>KQLRLYQLYSRTSGKHIQVLGRRISARGEDGDKYAQLLVETDTFGSQVRIKGKETEFYLCMNRKGKLVGKPDGTSKECVFIEKVLENNYTALMSAKYSGWYVGFTKKGRPRKGPKTRENQQDVHFMKRYPKGQPELQKPFK[4x]

Fibroblast growth factors (FGFs) regulate a plethora of critical processes in development. These processes are mediated by signaling through four FGF receptors (FGFR1–4), which are high-affinity cell surface receptor tyrosine kinases. FGF18 belongs to the paracrine-acting FGF8 subfamily, which contains three members in humans: FGF8, FGF17, and FGF18. FGF18 has a number of functions in the developing and adult organism including a key role in skeletal development and has undergone clinical trials for the treatment of osteoarthritis (Merck KGaA).

FGF18 was incubated stoichiometrically with heparin (6 dp) and the complex isolated prior to crystallization in a mother liquor of 0.1 mol/L MES pH 6.5, 0.2 mol/L ammonium sulphate and 26% PEG 5000. FGF18 crystallized in the primitive monoclinic spacegroup P21 with four FGF18 molecules in the asymmetric unit. The final model consists of residues 50–179 and has a β-trefoil core formed from ten anti-parallel β-strands arranged in three groups of three or four strands connected by tight turns and loops. There is a disulfide bridge between Cys109 and Cys127 that joins the β6 strand with the β7–β8 loop, helping to stabilize it. The four FGF18 molecules in the asymmetric unit have root mean-square deviation (RMSD) of 0.30 Å2 (Cα atoms). Differences are mainly at the crystal contact sites with greatest variation in the β4–β5 loop, residues 90–96, which in the FGF8 subfamily contains an extra serine residue that presumably increases its flexibility. Although electron density for heparin hexasaccharide is not present, 13 sulfate ions are discernable in the asymmetric unit, corresponding to 5 unique sulfate-binding locations. In our structure, sulfate ions are bound to the canonical binding site, but not to the proposed secondary site. Three of the five sulfate ions are clustered in a location distinct from the heparin-binding sites of FGF1/2, but occupy a continuous stretch of basic residues that is, in part, formed by the lysines identified as interacting with heparin by Xu et al. (2012), and could represent an extension of the canonical site. The model demonstrates how the extended and hydrophobic β4–β5 loop of FGF18 is important for conferring FGFR binding specificity as it engages the hydrophobic groove in the D3 domain of FGFR c-isoforms.>[2x]MSLFNDKVAKLLAGHEALLMRKNEPVEEGNGVITRYRYPVLTAAHTPVFWRYDLNEETNPFLMERIGMN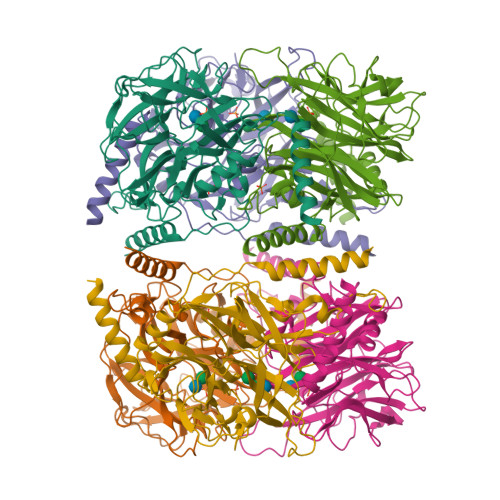ATLNAGAIKWDGKYLMLVRVEGADRKSFFAVAESPNGIDNFRFWEYPVTLPEDVVPATNVYDMRLTAHEDGWIYGIFCAERHDDNAPIGDLSSATATAGIARTKDLKNWERLPDLKTKSQQRNVVLHPEFVDGKYALYTRPQDGFIDTGSGGGIGWALIDDITHAEVGEEKIIDKRYYHTIKEVKNGEGPHPIKTPQGWLHLAHGVRNCAAGLRYVLYMYMTSLDDPTRLIASPAGYFMAPVGEERIGDVSNVLFSNGWIADDDGKVFIYYASSDTRMHVATSTIERLVDYCLHTPQDGFSSSASVEILKNLIERNLRLMK>MSFFHGVTVTNVDIGARTIALPASSVIGLCDVFTPGAQASAKPNVPVLLTSKKDAAAAFGIGSSIYLACEAIYNRAQAVIVAVGVETAETPEAQASAVIGGISAAGERTGLQALLDGKSRFNAQPRLLVAPGHSAQQAVATAMDGLAEKLRAIAILDGPNSTDEAAVAYAKNFGSKRLFMVDPGVQVWDSATNAARNAPASAYAAGLFAWTDAEYGFWSSPSNKEIKGVTGTSRPVEFLDGDETCRANLLNNANIATIIRDDGYRLWGNRTLSSDSKWAFVTRVRTMDLVMDAILAGHKWAVDRGITKTYVKDVTEGLRAFMRDLKNQGAVINFEVYADPDLNSASQLAQGKVYWNIRFTDVPPAENPNFRVEVTDQWLTEVLDVA[12x];>MIPQTLTNTNLFIDGVSFAGDVPSLTLPKLAVKTEQYRAGGMDAPVSIDMGLEAMEAKFSTNGARREALNFFGLADQSAFNGVFRGSFKGQKGASVPVVATLRGLLKEVDPGDWKAGEKAEFKYAVAVS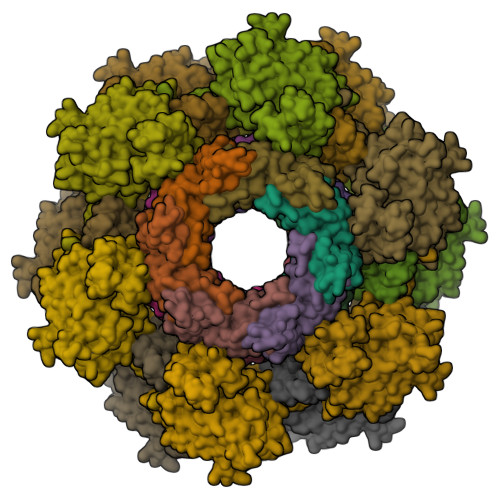YYKLEVDGREVYEIDPVNGVRAINGVDQLAGMRNDLGL[12x]>GPMADIGSLLQDSDSLSGSYLDPNYQSIKWQPHQQNKWATLYDANYKELPMLTYRVDADKGFNFSVGDDAFVCQKKNHFQVTVYIGMLGEPKYVKTPEGLKPLDCFYLKLHGVKLEALNQSINIEQSQSDRSKRPFNPVTV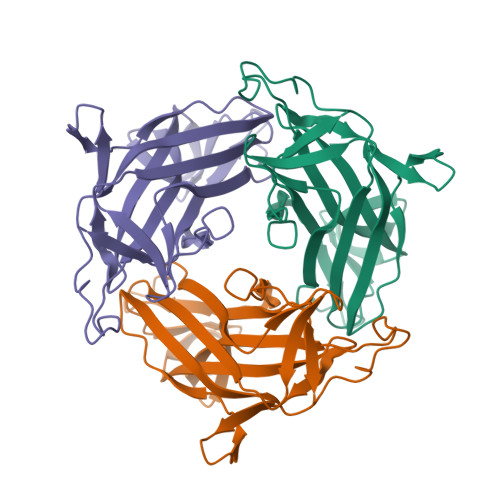NLPPEQVTKVTVGRLHFSETTANNMRKKGKPNPDQRYFMLVVALQAHAQNQNYTLAAQISERIIVRASNPGQFESDSDVLWQRAQVPDTVFHHGRVGINTDRPDEALVVHGNVK[2x]>EDICFIAGIGDTNGYGWGIAKELSKRNVKIIFGIWPPVYNIFMKNYKNGKFDNDMIIDKDKKMNILDMLPFDASFDTANDIDEETKNNKRYNMLQNYTIEDVANLIHQKYGKINMLVHSLANAKEVQKDLLNTSRKGYLDALSKSSYSLISLCKYFVNIMKPQSSIISLTYHASQKVVPGYGGGMSSAKAALESDTRVLAYHLGRNYNIRINTISAGPLKSRAATAINKLNNTYENNTNQNKNRNSHDVHNIMNNSGEKEEKKNSASQNYTFIDYAIEYSEKYAPLRQKLLSTDIGSVASFLLSRESRAITGQTIYVDNGLNIMFLPDDIYRNENE[2x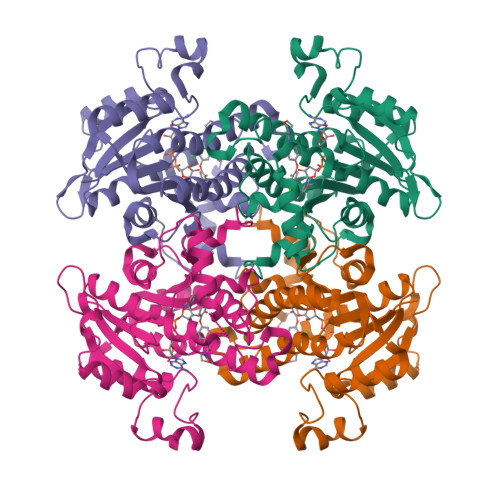]> SILVRRDAAPGASKLRAVLEKLKLSRDDISTAAGMVKGVVDHLLLRLKCDSAFRGVGLLNTGSYYEHVKISAPNEFDVMFKLEVPRIQLEEYSNTRAYYFVKFKRNPKENPLSQFLEGEILSASKMLSKFRKIIKEEINDIKDTDVIMKRKRGGSPA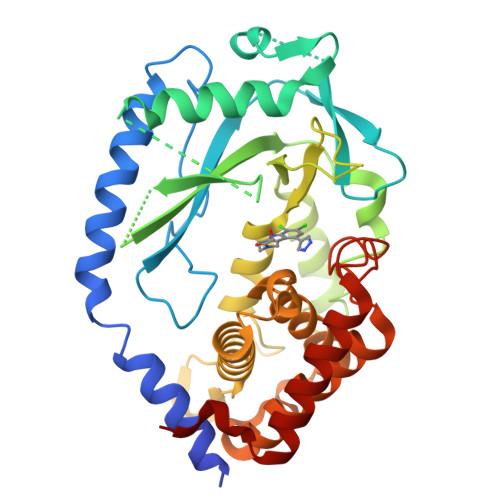VTLLISEKISVDITLALESKSSWPASTQEGLRIQNWLSAKVRKQLRLKPFYLVPKHAKEGNGFQEETWRLSFSHIEKEILNNHGKSKTCCENKEEKCCRKDCLKLMKYLLEQLKERFKDEEHLDKFSSYHVKTAFFHVCTQNPQDSQWDRKDLGLCFDNCVTYFLQCLRTEKLENYFIPEFNLFSSNLIDKRSKEFLTKQIEYERNNEFPVFDEF>MNRIKKVLVANRGEIAIRVMRACTELKIKTVAIYSQEDTGSFHRYKSDEAYLVGAGKKPIDAYLDIENIIEIAKESGADAIHPGYGFLSENIEFARRCEQEGIIFVGPKSKHLDMFGDKIKAKEQALLADIPVIPGSNGPVAGIKEVEEFGEKNGYPLMIKASLGGGGRGMRVVESKEHVKESFERASSEAKAAFGNDEVYVEKCVMNPKHIEVQILGDTHGNIVHLFERDCSIQRRHQKVVEVAPCNAITSELRNRICDAAVKLMKNVDYINAGTVEFLVEGDDFYFIEVNPRVQVEHTITEMITGIDIVQSQLFIADGYALHDQLVAIPKQEDIHIHGSAIQSRITTEDPLNNFMPDTGRVDTYRSTGGFGVRLDAGNGFQGTVVTPFYDSLLVKLCTWGMTFEQATRKMRRNLIEFRIRGVKTNIPFLLNVVRHPDFASGNYNTSFIDTTPELFKFPHIRDRGTKTLRYIGNVTVNGFPGIKHRDKPVYAEPRLPKIPYGSQISPGTKQILDAKGPEGVVDWVKKQEEVLLTDTTLRDAHQSLLATRVRSKDIFQIADAMAHLLPNMFSFEMWGGATFDVAYRFLNEDPWVRLETLRKQIPNVMFQMLLRGANAVGYKNYPDNVIREFVKQSAQSGVDVFRVFDSLNWIKGMEVSIDAVREAGKIVEAAICYTGDIDDDTRTKYTIDYYKDMAKELVAQGTHILGIKDMAGLLKPQAAYRLIGELKDTVDVPIHLHTHDTSGNGIYTYAAAVSAGVDIVDVASSAMSGATSQPSMTGLYYGLVNGNRQTNLDAQNSQIINHYWEDVRHYYKDFDNALNSPQTEVYIHEMPGGQYTNLQQQAIAVGLGDRWDEVKEMYTVVNQMFGDIVKVTP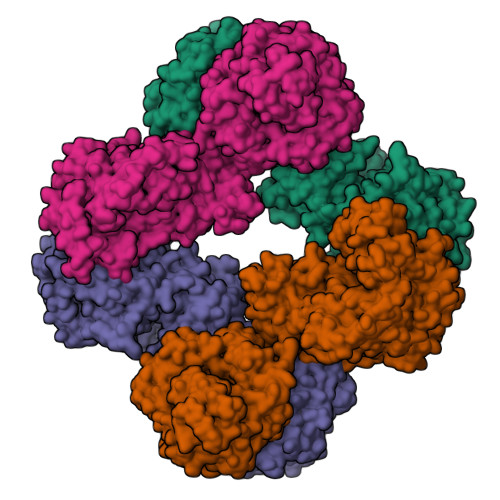SSKVVGDLALFMVQNELSEEDVYEKGDTIDFPDSVIEFFMGEIGQPYGGFPEKLQKLVLKGRTPLTDRPGALMEPVNFVEVKAELKEKMGYEPTEKDVISYILYPKVFLDYQEMINKYGDVTVLDTPTFYKGMRLGETIEVELEKGKILLIKLNSIGEPIADGTRVIYFELNGQPREINIQDMNVQSTVIARRKIDTTNPEHVGATMTGSVIQVVVKKGDSVKKGDPLLITEAMKMETTIQAPFDGEVSSIYVSDGDTIESGDLLIEVNRI[8x]>[4x]SGRTWREADINYTSGFRNSDRILYSSDWLIYKTTDHYQTFTKIRCAQVINTFDGVADYLQTYHKLPDNYITKSEAQALGWV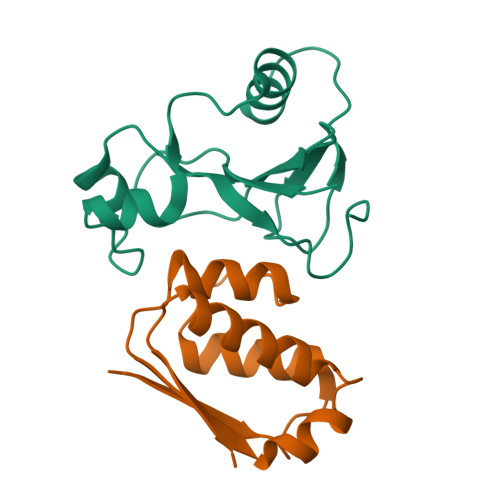ASKGNLADVAPGKSIGGDIFSNREGKLPGK;>[4x]MKKAVINGEQIRSISDLHQTLKKELALPEYYGENLDALWDCLTGWVEYPLVLEWRQFEQSKQLTENGAESVLQVFREAKAEGCDITIILS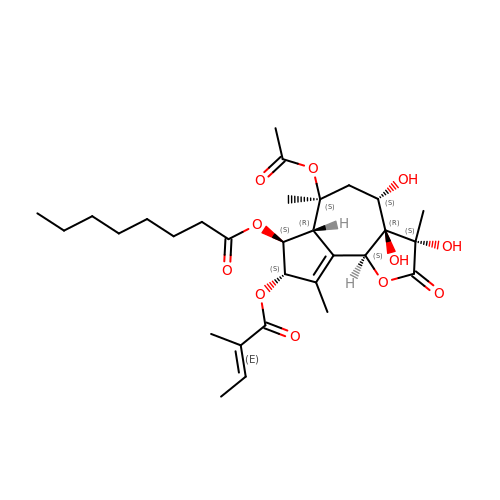DEBUTANOYL THAPSIGARGIN | C30 H44 O11 | UBPDDZPGODTCDF-NPAVTDDVSA-N> MSRCGSLGLYAPNALPSLSLKPRSVKSPFCITSHTKPNDTLLHNVNKMRAKACDILGAKKTILAAQLGAVLATIDHPALAITGVNNQQELSSVVLDIGIISVWYFLVMPPIIMNWLRVRWYRRKFFEMYLQFMFVFMFFPGLLLWAPFLNFRKFPRDPNMKNPWDKPTDPDSIK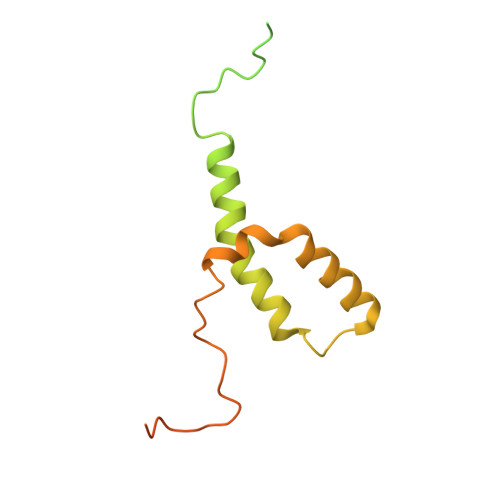NVYLKYPYATPEDYDLD The essential enzyme messenger RNA (mRNA) (guanine-N7) methyltransferase catalyzes S-adenosylmethionine (SAM)-dependent conversion of GpppRNA ends to the m7GpppRNA cap structure characteristic of eukaryal mRNAs. The antibiotic sinefungin (SFG) is a SAM analog in which the S-CH3 sulfonium moiety of SAM is replaced by a C-NH2 amine. Available evidence indicates that the antifungal activity of SFG is exerted via inhibition of fungal cap methyltransferase Abd1. Crystal structures of K. lactis and S. cerevisiae Abd1 as binary complexes with SAH or SFG and ternary complexes with GTP•SFG highlight how SFG makes two hydrogen bonds from its C-NH2 amine to the guanine-O6 and -N7 atoms of GTP that account for its higher affinity vis-à-vis SAH and SAM.

To elucidate the role of Tyr416 substitutions in ScAbd1 in conferring SFG resistance, ScAbd1Δ140-K163R-K311R-F387Y-Y416F was purified and co-crystallized in the presence of 1 mM SFG and 3 mM GTP. The structure was refined at a resolution of 2.8 Å with Rwork/Rfree of 18.2/21.7. The crystals contained three ScAbd1 complexes in the asymmetric unit and the tertiary structures of the protomers are very similar to each other (r.m.s.d. between 0.21 and 0.25 Å over 256 Cα positions). SFG engages with the same ensemble of enzymic residues observed in the wild-type ScAbd1•SFG•GTP structure and the C-NH2 amine of SFG makes hydrogen bonds with the O6 (2.9 Å) and N7 (2.5 Å) atoms of GTP, à la the wild-type structure. Whereas the GTP contacts in the SFG-resistant ScAbd1 recapitulate many of those seen in the wild-type ternary complex, there are some noteworthy differences. First, only one of the Glu347 carboxylate oxygens is coordinating the guanine-N1 (2.8 Å) and -N2 (3.2 Å) atoms. Second, there is no contact between His253 and guanine-O6 in the variant complex. Third, and most relevant, the Tyr416 phenolic hydroxyl-mediated polar contacts with the guanine-N3 and ribose-O2′ atoms of GTP observed in the wild-type active site are missing in the SFG-resistant variant in which Tyr416 is changed to Phe. Absence of the two hydrogen bonds between GTP and Tyr416 is likely to reduce the cap binding affinity of the SFG-resistant variants. In addition, whereas the electron densities for Phe416 and SFG in the resistant variant are well defined, the density for GTP is relatively weak, specifically around the guanosine and ribose moieties, when compared to the GTP density in the wild-type ternary complex.

>[3x]SPIIKLRNFNNAIKYMLIDKYTRPGDVVLELGCGKGGDLRKYGAAGISQFIGIDISNASIQEAHKRYRSMRNLDYQVVLITGDCFGESLGVAVEPFPDCRFPCDIVSTQFCLHYAFETEEKARRALLNVAKSLKIGGHFFGTIPDSEFIRYKLNKFPKEVEKPSWGNSIYRVTFENNSYQKNDYEFTSPYGQMYTYWLEDAIDNVPEYVVPFETLRSLADEYGLELVSQMPFNKFFVQEIPKWIERYSPKMREGLQRSDGRYGVEGDEKEAASYFFTMFAFRKVKQYIEPESVKPN> SSAANAYNAG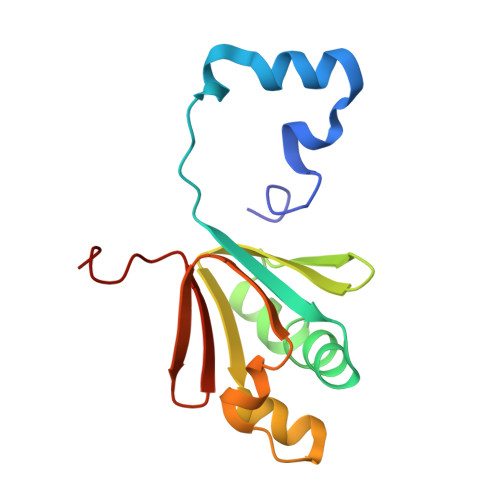IMQKTGKAFADEFFAEENQVVHESNAVVLVLMKSDEIDAIIEDIVLKGGKAKNPSIVVEDKAGFWWIKADGAIEIDAAEAGELLGKPFSVYDLLINVSSTVGRAYTLGTKFTITSELMGLDR>[4x]VLDGPYQPTNFKPPNDYWILLNPTNQQVVLEGTNKTDIWVALLLVEPNVTNQSRQYTLFGETKQITVENNTNKWKFFEMFRSNVSAEFQHKRTLTSDTKLAG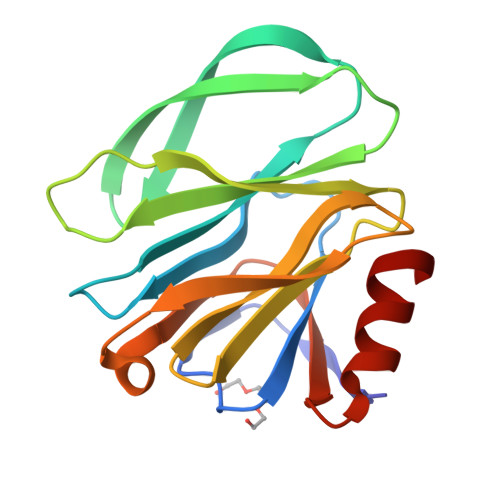FMKFYNSVWTFHGETPHATTDYSSTSNLSEVETVIHVEFYIIPRSQESKCSEYINTGL>[2x]DDLYRQSLEIISRYLREQATGSKDTKPLGEAGAAGRRALETLRRVGDGVQRNHETAFQGMLRKLDIKNEDDVKSLSRVMIHVFSDGVTNWGRIVTLISFGAFVAKHLKTINQESCIEPLAESITDVLVRTKRDWLVKQRGWDGFVEFFHVEDLE

Three subsets of Bcl-2 proteins interact to determine whether cells commit to apoptosis. The BH3-only proteins then associate with anti-apoptotic Bcl-2 relatives (Mcl-1, Bcl-2, Bcl-xL, Bcl-w, Bfl-1/A1, Bcl-b) preventing their binding and inactivation of Bak and Bax (effector Bcl-2 proteins) which can then form oligomeric pores at the outer mitochondrial membrane causing cytochrome c release and caspase activation. Although the pro-survival Bcl-2 family members share several functions and structural features, the distinctive regulation of Mcl-1 makes this anti-apoptotic protein unique. Mcl-1 has attracted attention because of its established role in preventing cell death by binding and sequestering pro-apoptotic BH3 proteins, thereby mediating cancer cell survival, as well as intrinsic and acquired resistance against cytotoxic and some targeted therapies, including venetoclax.

One avenue began with analysis of a series of indole-2-carboxylic acids which have been reported by others. Investigating one such literature compound, 1, we were able to obtain a co-crystal structure in complex with Mcl-1. Surprisingly, we observed two inhibitors bound to the BH3-binding domain of Mcl-1. The first high-affinity binding (cyan molecule in Fig. 1a) overlays well with reported crystal structures, with the 2-carboxylic acid forming an ionic interaction with Arg263 of Mcl-1 (dotted line) and the naphthyl group occupying an induced-fit pocket. To our knowledge, this 2:1 stoichiometry has not been observed previously with this series of compounds and results in a conformational change in Mcl-1 protein residues (e.g., Met231 side chain and larger movement in the Leu246 to Asp256 helix) to enlarge the binding pocket and accommodate the second binding molecule. Since this larger pocket may be more druggable, we hypothesized that a new hybrid molecule able to take advantage of both binding events would have vastly improved potency compared to 1 or 2 (Mcl-1 TR-FRET IC50s = 1.1 and 0.29 µM, respectively). Given the short distance between these molecules, we reasoned that a two-atom linker would be appropriate to link the two monomers. Application of structure-based drug design to a new binding mode of a known inhibitor scaffold bound to Mcl-1 led to identification of an induced-fit pocket in Mcl-1.> MGDTKEQRILRYVQQNAKPGDPQSVLEAIDTYCTQKEWAMNVGDAKGQIMDAVIREYSPSLVLELGAYCGYSAVRMARLLQPGARLLTMEINPDCAAITQQMLNFAGLQDKVTILNGASQDLIPQLKKKYDVDTLDMVFLDHWKDR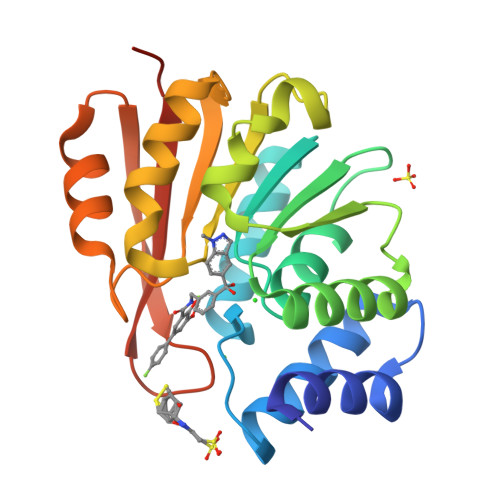YLPDTLLLEKCGLLRKGTVLLADNVIVPGTPDFLAYVRGSSSFECTHYSSYLEYMKVVDGLEKAIYQGPSSPDKS>MMKKADSVPTPAEAALAAQTALAADDSPMGDAARWAMGLLTSSGLPRPEDVAARFIPTFAAAGNFAETVREWRSKGPFTVRAYHPVAHKGWVVLSAPAGVRYILSLTLDSSGLIRILTLKPETVIPDMVTWNDVEETLHTPGVQHSVYAVRLTPDGHEVLHASAPERPMPTGAAYKLYLMRALVAEIEKGTVGWDEILTLTPELRSLPTGDMQDLPDGTRVTVRETAHKMIALSDNTGADLVADRLGREVVERSLAAAGHHDPSLMRPFLTSHEVFELGWGDPERRAEWVRQDEAGRRELLEKMAGVMTVRGSDLGATVHQLGIDWHMDAFDVVRVLEGLLQDSGR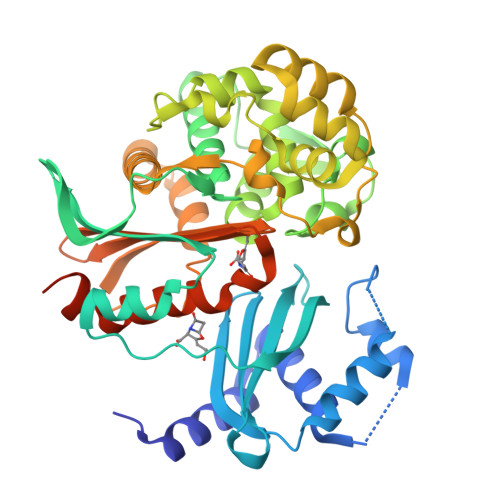DTSGTVEEILTAYPGLLIDEERWRRVYFKAGSSPGVMMFCWLLQDHAGISYVLVLRQSADEQRLIGDGLFLRGIGAKIIEAEAKLLSSGERRGAGTAAAGDDRASAGEAARR[2x]>[4x]MAHHHHHHMRDAPASMPRVDGDRLWASLERMAQIGATPKGGVCRLALTDLDRESRDLFVQWAREAGCTVRVD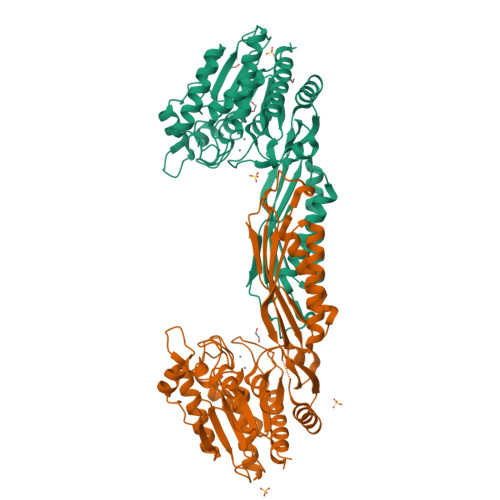RMGNVFARRAGRRPDAAPVMTGSHADSQPTGGRYDGIYGVLGGLEVVRALNDAAIETERPVDVVIWTNEEGSRFAPAMVSAGVFSGVYTLEYGLSRTDGAGRTIGEELERIGYAGAEPVGGYPVHAAYELHIEQGAILERAGKTIGVVTAGQGQRWYEVTLTGVDAHAGTTPMAFRRDALVGAARMISFVEVLGRRYAPDARATVGMIEARPNSRNTVPGGCFFTVEFRHPDDAVLDELDAALRAELARVADETGLGAQIEQIFTYAPVPFAPRCIDTVRDAARSLGLSHMDIVSGAGHDACYVARVAPTGMIFVPCVDGLSHNEAEAITPEWATAGADVLLRAVLQSAQEA> MSQSTASLVPEGNQGSLQEDVSFDFNGVPGQALDAVRMRLAQLTHSLRRIRDEMSKAELPQWYTLQSQLNVTLSQLVSVTSTLQHFQETLDSTVVYPLPKFPTTSHESLVTTLLRKKNIPEVDEWMKYVRETSGVTTALLKDEE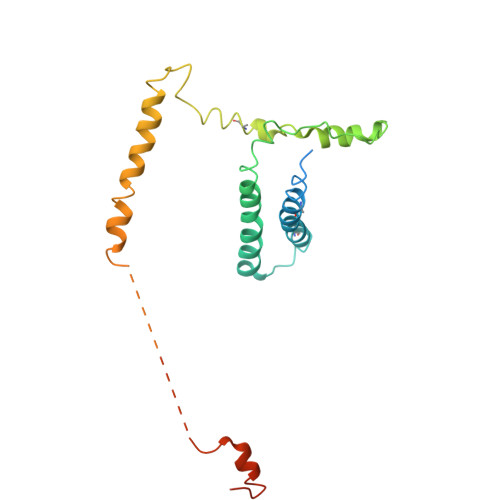IEKLLQQDREITNWARTTFRNEYGKHDFKNEESLSEEHASLLVRDSKPSKPFNVDDVLKFTFTGEKPIITGSTSTSSSN>HGYVSSPKSRVIQCKENGIENPTHPACIAAKAAGNGGLYTPQEVAVGGVRDNHDYYIPDGRLCSANRANLFGMDLARNDWPATSVTPGAREFVWTNTAAHKTKYFRYYITPQGYDHSQPLRWSDLQLIHDS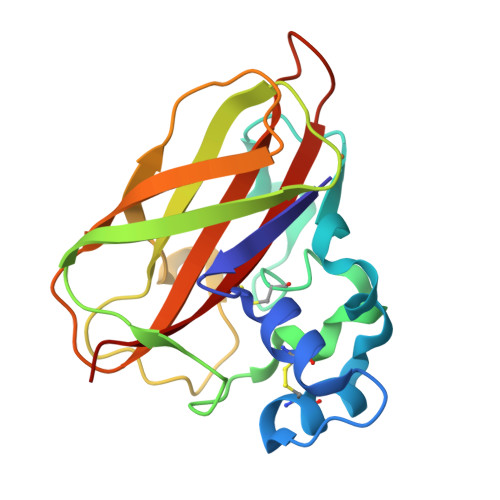GPADQEWVSTHNVILPYRTGRHIIYSIWQRDWDRDAAEGFYQCIDVDFG[3x]Several sets of host cell machinery facilitate this process, including proteins of the endosomal sorting complexes required for transport pathway, which mediates the membrane fission reaction required to complete viral budding, as well as angiomotin (AMOT) and NEDD4L, which bind one another and promote virion membrane envelopment. AMOT and NEDD4L interact through the four NEDD4L WW domains and three different AMOT Pro-Pro-x (any amino acid)-Tyr (PPxY) motifs, but these interactions are not yet well defined. Here, we report that individual AMOT PPxY and NEDD4L WW domains interact with the following general affinity hierarchies: AMOT PPxY1>PPxY2>PPxY3 and NEDD4L WW3>WW2>WW1∼WW4. Comparative structural, binding, and virological analyses reveal that complementary ionic and hydrophobic contacts on both sides of the WW–PPxY core interaction account for the unusually high affinity of the AMOT PPxY1–NEDD4L WW3 interaction.

To obtain structures, we screened a series of different high- and moderate-affinity AMOT PPxY–NEDD4L WW complexes for crystallization. Two such complexes, AMOT PPxY2–NEDD4L WW1 and AMOT PPxY2–NEDD4L WW2, yielded high-resolution crystal structures (1.52 Å and 1.74 Å, respectively). All five of our new structures exhibit canonical WW domains, with three-stranded β-sheets and canonical positioning of the two eponymous Trp residues. In all three WW–PPxY complexes, the PPxY core elements bind in an extended polyproline II helical conformation across the concave WW sheet. Each conserved residue in the PPxY motif makes canonical binding interactions: the first Pro/Leu residue binds in the “XP-groove,” where it stacks against the second conserved WW Trp residue (Trp525 in WW3). The second PPxY Pro packs against a Tyr/Phe residue from the second β-strand (β2), and its carbonyl oxygen forms a hydrogen bond to the hydroxyl of a conserved Thr (in β3). The fourth Tyr residue of PPxY binds in the characteristic “Y-pocket”, forming a hydrogen bond with conserved His (in loop-II between β2 and β3). In contrast, the PPxY2–WW1 and PPxY2–WW2 complexes make few favorable contacts outside the core. On the N-terminal side, the PPxY1 backbone approaches WW3 loop-I more closely (∼6 Å) than PPxY2 in the WW1 or WW2 complexes (11 Å and 14 Å, respectively).

>[3x]QPHMPGLPSGWEERKDAKGRTYYVNHNNRTTTWTRPIM;>MEHRGPPPEYPFKGM[3x]Aconitase superfamily members catalyze the homologous isomerization of specific substrates by sequential dehydration and hydration and contain a [4Fe-4S] cluster. However, monomeric and heterodimeric types of function unknown aconitase X (AcnX) have recently been characterized as a cis-3-hydroxy-L-proline dehydratase (AcnXType-I) and mevalonate 5-phosphate dehydratase (AcnXType-II), respectively. We herein elucidated the crystal structures of AcnXType-I from Agrobacterium tumefaciens (AtAcnX) and AcnXType-II from Thermococcus kodakarensis (TkAcnX) without a ligand and in complex with substrates. AtAcnX and TkAcnX contained the [2Fe-2S] and [3Fe-4S] clusters, respectively, conforming to UV and EPR spectroscopy analyses.

To clarify substrate binding, we directly co-crystallized the wild-type enzyme of TkAcnX (inactive form) with MVA5P, and the crystal structure was elucidated at a resolution of 1.9 Å. The [3Fe-4S] cluster was located at the same position as the structure of the apo-form, and additional electron density around the [3Fe-4S] was clearly modeled as MVA5P. In the structure of the holo-form, TkAcnXS and TkAcnXL showed no large conformational changes from those in the apo-form (chains D and C); r.m.s.d. values on Cα atoms were 0.5 and 0.6 Å, respectively. On the other hand, the two subunits were closely rotated by an angle of ~26°; substrate binding resulted in a more “closed” conformation than the structure in the apo-form. The carboxyl group of bound MVA5P made hydrogen bond(s) and/or salt bridge(s) with the side chains of Thr63(S), Ser130(L), and Lys361(L), the main chain nitrogen atoms of Thr63(S) and Ser130(L), and a water molecule. The water molecule further interacted with the side chain of Tyr365(L). The hydroxyl group of MVA5P on C3 formed hydrogen bonds with the side chains of Glu129(L) and Lys361(L), among which the former interacted with the side chains of Asn79(L) and Ser131(L). The 5-phosphate group made hydrogen bonds with the main chain nitrogen atoms of Gly48(L), Val49(L), and Ser50(L), and the side chains of Asn53(L) and Asn79(L). In addition, Ser62(S) was close to C2 of MVA5P (a distance of 3.2 Å) and superimposed onto Ser70 in AtAcnX. Therefore, the catalytic mechanism of TkAcnX may be similar to that of AtAcnX, except for the involvement of the [4Fe-4S] cluster as a Lewis acid instead of the [2Fe-2S] cluster.

> MYLTKEEELILAGEYGYALQKAMEILVALGDIYGADRLIPIKSAQVAGVSYKNIGDAGIEFLRDFVEAGAKVSVYTTLNPAGIGDDEFMEKQMEVLELYRKMGIEVTSTCTPYYGANLPKFGDHIAWSESSAVSFANSILGARTNREGGPSSLAAAIVGKTPNYGLHLDENRKATVIVDVKAKVKTFADYSVLGYHVGKTLGNDVPYFKNLKPEKTEFLKELGAAMGATGSIALYHVEGETPEYREAITDKLETITVEDSDLKAVRESFQDDWSDIDMILIGCPHASLPEVKEIAELLRMRGKPLKIPLFITASRAVKALADALGYTEIIERYNGKIIPDSCFVVSPIKGWYRGIATNSGKSAFYFRSFGFSVRLDDVENLIKEAP;> GPKLKGRKIVGGKAEGEVIVSRKPLSFLGGVDPETGIVTDAESDIRGQSIAGKILVFPRGKGSTVGSYVIYALKKNNKAPKAIIVGEAETIVATGAIISDIPMVDGVDVSKLKTGMKVRVDADSGEVEILEDGE>[4x]SNALSIDEAFRKFKSRLELNEREQKNASQRQNEVRDYLQTKFGIARSFLTGSYARYTKTKPLKNINIFFVLKDS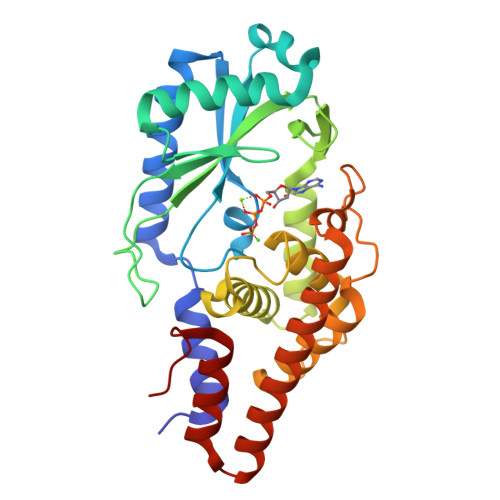EKHYHGKAASVVLDDFHSALVEKYGSAAVRKQARSINVDFGVHIDAEDNTDYRVVSVDAVPAFDTGDQYEIPDTASGKWIKTDPEIHKDKATAAHQAYANEWKGLVRMVKYWNNNPKHGDLKPVKPSFLIEVMALECLYGGWGGSFDREIQSFFATLADRVHDEWPDPAGLGPAISNDMDAARKQRAQQLLFQASQDASIAIDHARRGRNIEALRAWRALFGPKFPLS> MLATPFYSRSDRIFGIVNAVLLGIFALCALYPIIYIFSMSISSGAAVTQGRVFLLPVDIDFSAYGRVLHDKLFWTSYANTIFYTVFGVVTSLIFIVPGAYALSKPRIRGRRVFGFIIAFTMWF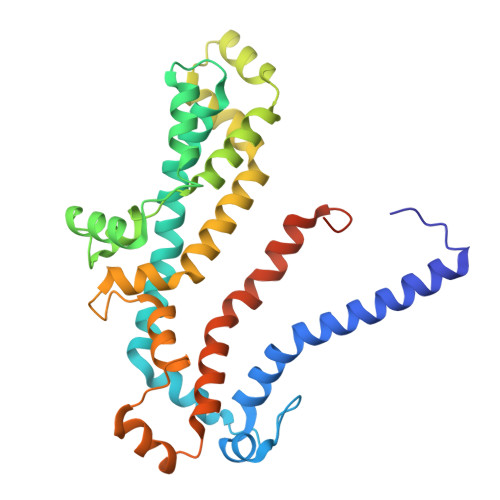NAGMIPFFLNMRDLGLLDNRFGILIGFACNAFNIILMRNYFESISASFEEAARMDGANDLQILWKVYIPLAKPALATITLLCAISRWNGYFWAMVLLRAEEKIPLQVYLKKTIVDLNVNEEFAGALLTNSYSMETVVGAIIVMSIIPVIIVYPVVQKYFTKGVMLGGVKELEHHHHHHHHHH>HHHHHHLEVLFQGPMKYTKLEKDALDLLSDNEEEDAESSILTFEERDTSSLSIEARLESIEEKLSMILGLLRTLNIATAGPTAARDGIRDAMIGVREEL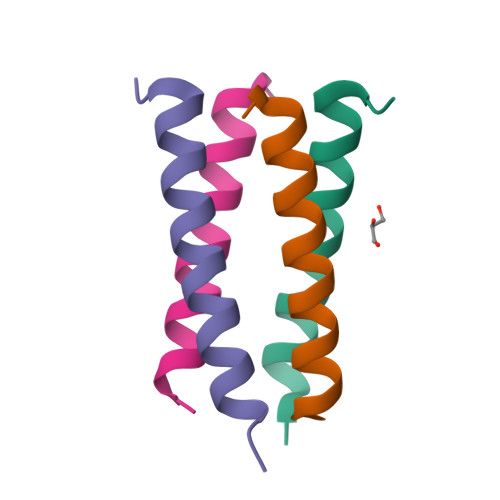IADIIKEAKGKAAEMMEEE[8x]> MSAFPDSMDQKFHNMTVNECFQSRSTVLQGQPFGGIPTVLVLNIILWVFVVLLYSFLRKAAWDYGRLALLIHNDSLTSLIYGEQSEKSSPSEVSLEAERRDRGFSSWFFNSLTMRDRDLINKCGDDARIYITFQYHLIIFVLILCIPSLGIILPVNYIGTVLDWNSHFGRTTIVNVSTESKFLWLHSLFAFLYFLINLAFMGHHCLGFVPKKSLHFTRTLMITYVPTEIQDPEIISKHFH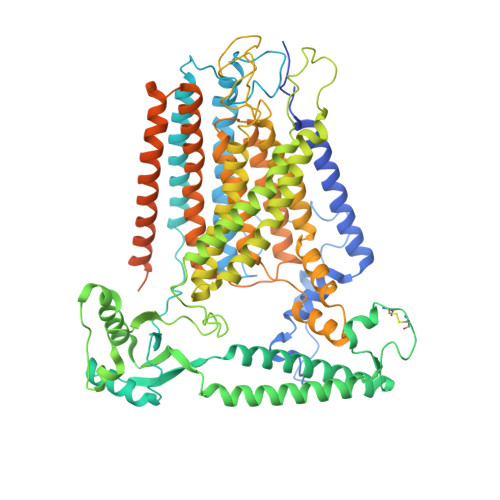EAYPGCVVTRVHFCYDVRNLIDLDDQRRHAMRGRLYYTAKAKKTGKVMIKTHPCSRLCFCKCWTCFKEVDAEQYYSELEEQLTDEFNAELNRVQLKRLDLIFVTFQDARTVRRIYDDYKYIHCGRHPKQSSVTTIVKNYHWRVAHAPHPKDIIWKHLSIRRFSWWTRFIAINTFLFFLFFFLTTPAIIINTIDIYNVTRPIEKLQSPIVTQFFPSVLLWAFTVTMPLLVYLSAFLEAHWTRSSQNLIIVHKCYIFLVFMVVILPSMGLTSLHVFLRWLFDIYYLEHATIRFQCVFLPDNGAFFINYVITAALLGTGMELMRLGSLCTYCTRLFLSKSEPERVHIRKNQATDFQFGREYAWMLNVFSVVMAYSITCPIIVPFGLLYLCMKHITDRYNMYYSYAPTKLNAQIHMAAVYQAIFAPLLGLFWMLFFSILRVGSLHSITLFSMSSLIISVVIAFSGVFLGKLRIAQRYEQPEEETETVFDVEPSSTTSTPTSLLYVATVLQEPELNLTPASSPARHTYGTINSQPEEGEEESGLRGFARELDSAQFQEGLEMEGQSH>[4x]SNAEDELYRQSLEIISRYLREQATGAKDTKPMGRSGATSRKALETLRRVGDGVQRNHETAFQGMLRKLDIKNEDDVKSLSRVMIHVFSDGVTN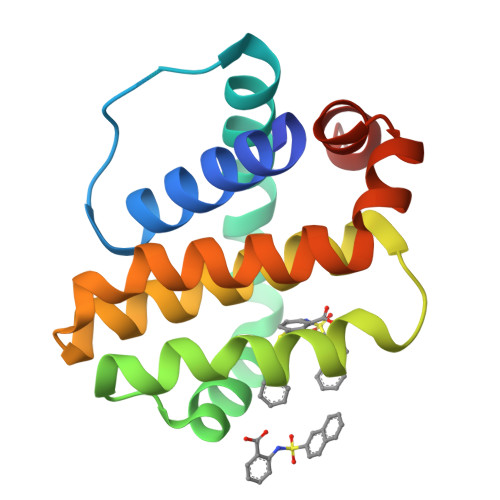WGRIVTLISFGAFVAKHLKTINQESCIEPLAESITDVLVRTKRDWLVKQRGWDGFVEFFHVED> MYIDQHNGVDMGVDLKDIIPGEAKTVIEDLRILHGKIIVIDGYNALYQFLAAIRQPDGTPLMDNNGRITSHLSGLFYRTINIVEAGIKPVYVFDGKPPELKAREIERRKAVKEEAAKKYEEAVQSGDLELARRYAMMSAKLTEEMVRDAKSLLDAMGIPWVQAPAEGEAQAAYIVKKGDAYASASQDYDSLLFGSPKLVRN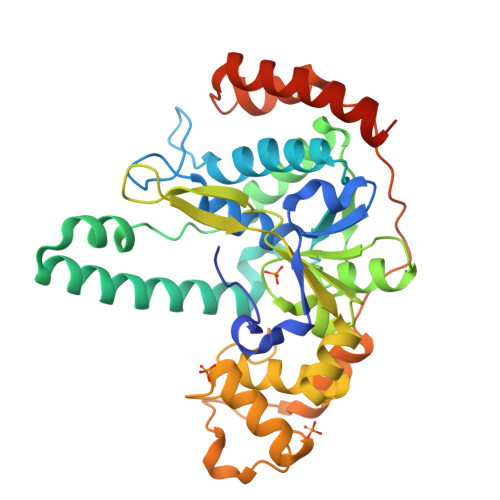LTISGRRKLPRKNEYVEVKPELIELDKLLVQLGITLENLIDIGILLGTDYNPDGFEGIGPKKALQLVKAYGGIEKIPKPILKSPIEVDVIAIKKYFLQPQVTDNYRIEWHTPDPDAVKRILVDEHDFSIDRVSTALERYVKAFKENIRGEQKGLSKWFSKPK>MKITNPVLKGFNPDPSICRA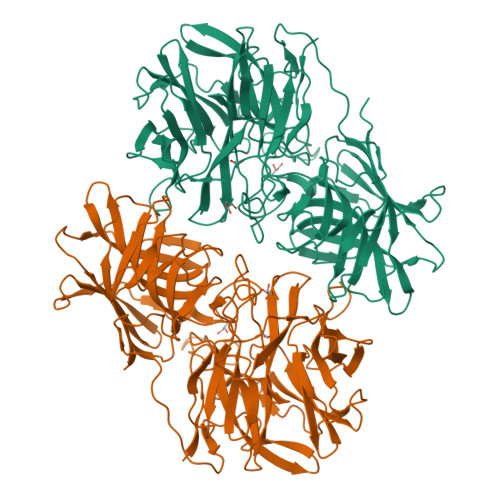GEDYYMAVSTFEWFPGVQIYHSKDLIHWRLAARPLQKTSQLDMKGNPDSGGVWAPCLSYADGQFWLIYSDIKVVDGPFKDGHNYLVTADAVDGEWSDPVRLNSSGFDPSLFHDPSGKKYVLNMLWDHREKHHSFAGIALQEYSVSEKKLVGERKVIFKGTPIKLTEAPHLYYINDVYYLLTAEGGTRYEHAATIARSSRIDGPYEVHPDNPILTAFHAPSHPLQKCGHASIVQTHTNEWYLAHLTGRPIHSSKESIFQQRGWCPLGRETAIQKLEWKDGWPYVVGGKEGLLEVEAPAMSVKEFSPTYHIVDEFKDSSLNRHFQTLRIPFTDQIGSVTENPHHLRLYGQESLTSKFTQAFVARRWQSFYFEAETAVSFFPKNFQQAAGLVNYYNTENWTALQVTYDDALGRILELSVCENLAFSQPLIKKIIIPDEIPYVYLKVTVQRETYTYSYSFDQQEWEKIDVPLESTHLSDDFIRGGGFFTGAFVGMQCQDTSGERLPADFKYFRYEETTEHHHHHH[2x]1-palmitoyl-2-oleoyl-sn-glycero-3-phosphoinositol 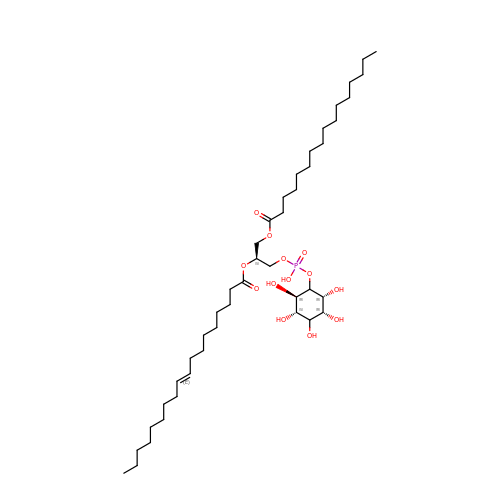| C43 H81 O13 P | PDLAMJKMOKWLAJ-QDJAQJDBSA-N(3aR,5R,6R,7R,7aR)-5-(hydroxymethyl)-2-methyl-5,6,7,7a-tetrahydro-3aH-pyrano[3,2-d][1,3]thiazole-6,7-diol 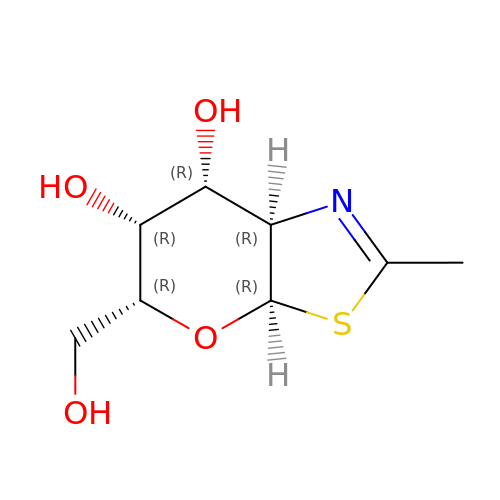| C8 H13 N O4 S | DRHXTSWSUAJOJZ-JAJWTYFOSA-N> MLRPVETPTREIKKLDGLWAFSLDRENCGIDQRWWESALQESRAIAVPGSFNDQFADADIRNYAGNVWYQREVFIPKGWAGQRIVLRFDAVTHYGKVWVNN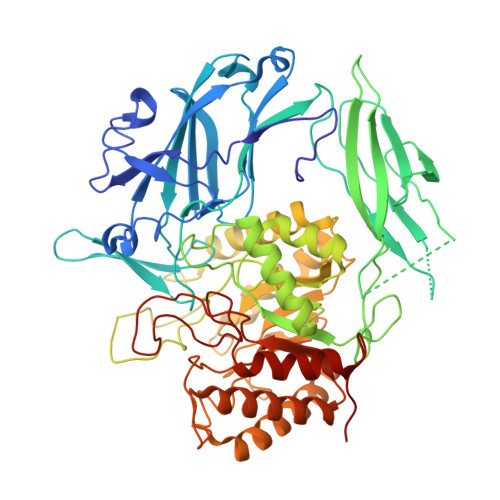QEVMEHQGGYTPFEADVTPYVIAGKSVRITVCVNNELNWQTIPPGMVITDENGKKKQSYFHDFFNYAGIHRSVMLYTTPNTWVDDITVVTHVAQDCNHASVDWQVVANGDVSVELRDADQQVVATGQGTSGTLQVVNPHLWQPGEGYLYELCVTAKSQTECDIYPLRVGIRSVAVKGEQFLINHKPFYFTGFGRHEDADLRGKGFDNVLMVHDHALMDWIGANSYRTSHYPYAEEMLDWADEHGIVVIDETAAVGFNLSLGIGFEAGNKPKELYSEEAVNGETQQAHLQAIKELIARDKNHPSVVMWSIANEPDTRPQGAREYFAPLAEATRKLDPTRPITCVNVMFCDAHTDTISDLFDVLCLNRYYGWYVQSGDLETAEKVLEKELLAWQEKLHQPIIITEYGVDTLAGLHSMYTDMWSEEYQCAWLDMYHRVFDRVSAVVGEQVWNFADFATSQGILRVGGNKKGIFTRDRKPKSAAFLLQKRWTGMNFGEKPQQGGKQ>ATPHINAEMGDFADVVLMPGDPLRAKYIAETFLEDAREVNNVRGMLGFTGTYKGRKISVMGHGVGIPSCSIYTKELITDFGVKKIIRVGSCGAVLPHVKLRDVVIGMGACTDSKVNRIRFKDHDFAAIADFDMVRNAVDAAKALGIDARVGNLFSADLFYSPDGEMFDVMEKYGILGVEM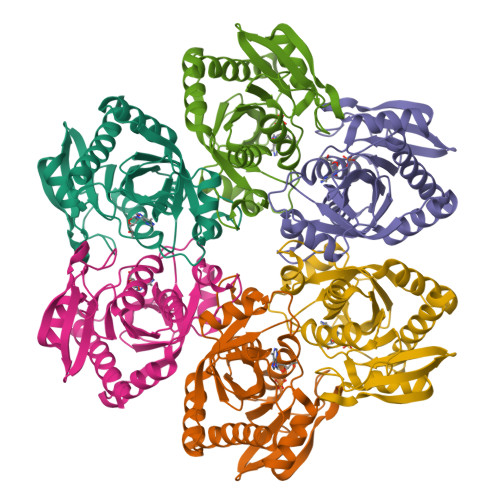EAAGIYGVAAEFGAKALTICTVSDHIRTHEQTTAAERQTTFNDMIKIALESVLLGDKE[3x]> MGHHHHHHHHHHSSGHIDDDDKHMSKKEININNYNDDAIQVLEGLDAVRKRPGMYIGSTDGAGLHHLVWEIVDNAVDEALSGFGDRIDVTINKDGSLTVQDHGRGMPTGMHAMGIPTVEVIFTILHAGGKFGQGGYKTSGGLHGVGSSVVNALSSWLEVEITRDGAVYKQRFENGGKPVTTLKKIGTAPKSKTGTKVTFMPDATIFSTTDFKYNTISERLNESAFLLKNVTLSLTDKRTDEAIEFHYENGVQDFVSYLNEDKEILTPVLYFEGEDNGFQVEVALQYNDGFSDNILSFVNNVRTKDGGTHETGLKSAITKVMNDYARKTGLLKEKDKNLEGSDYREGLAAVLSILVPEEHLQFEGQTKDKLGSPLARPVVDGIVADKLTFFLMENGELASNLIRKAIKARDAREAARKARDESRNGKKNKKDKGLLSGKLTPAQSKNPAKNELYLVEGDSAGGSAKQGRDRKFQAILPLRGKVINTAKAKMADILKNEEINTMIYTIGAGVGADFSIEDANYDKIIIMTDAD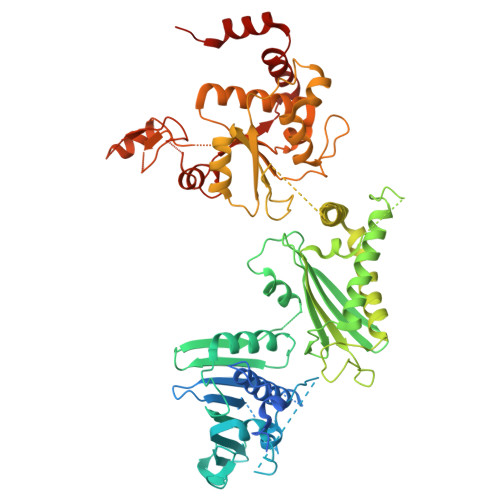TDGAHIQTLLLTFFYRYMRPLVEAGHVYIALPPLYKMSKGKGKKEEVAYAWTDGELEELRKQFGKGATLQRYKGLGEMNADQLWETTMNPETRTLIRVTIEDLARAERRVNVLMGDKVEPRRKWIEDNVKFTLEEATVF> MLYGVEIDEQYLRVMEEYKDKEVITQADMAKVALQRKNVYQDQAEKRQAELKAEYGVGVCVLVRVYNATGGPITAKIE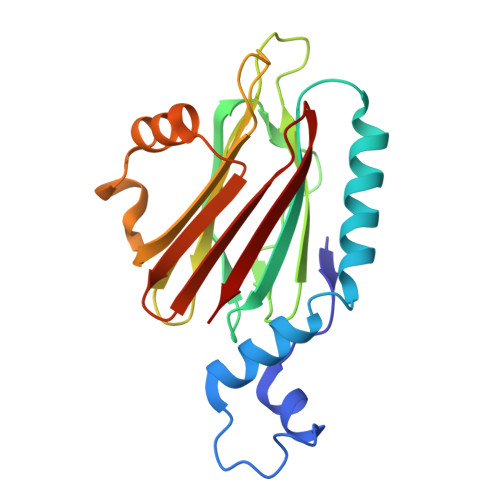ESFRGHFGAHTREKRIGNGQWTVFIHTKSAGAAVGSAGCIVYGTTDNLDIFSGWQNPWNRSWDSQVLVEVRQSGHWWKNGSKDYMLHLLDTHNGQNSDSSYGDVKAHGSTGNETTAYVEYVYSR>[2x]MGAAPDSHQLAKALAEAADVGAQMIKLVGLRELSEAERQLRSLVVALMQEVFTEFFPGCVVHPFGSSINSFDVHGCDLDLFLDLGDLEEPQPVPKLPPASPLLEDREEGDLGKASELAETPKEEKAEGAAMLELVGSILRGCVPGVYRVQTVPSARRPVVKFAHRPSGLHGDVSLSNRLALHNSRFLSLASELDGRVRPLVYTLRAWAQGRGLSGSGPLLSNYALTLLVIYFLQTRDPPVLPTVSQLTQKAG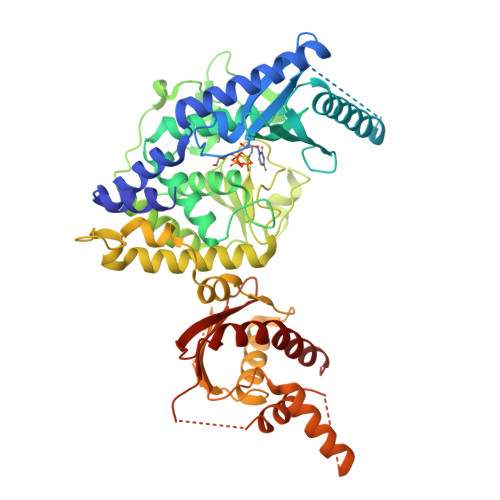EGEQVEVDGWDCSFPRDASRLEPSINVEPLSSLLAQFFSAVSSWDLRGSLLSLREGQALPVAGGLPSNLWEGLRLGPLNLQDPFDLSHNVAANVTSRVAGRLQNCCRAAANYARSLQYQRRSSRGRDWGLLPLLQPSSPSSLLSATPIPLPLAPFTQLTAALVQVFREALGCHIEQATKRTRSEGGGTGQGEAGKGASLPSSASWRCALWHRVWQGRRRARRRLQQQTKEGAGGGAGTRAGWLATEAQVTQELKGLSGGEERPETEPLLSFVASVSPADRMLTVTPLQDPQGLFPDLHHFLQVFLPQAIRHLKLEHHHHHH5-methoxy-2-methyl-1H-indole | C10 H11 N O | 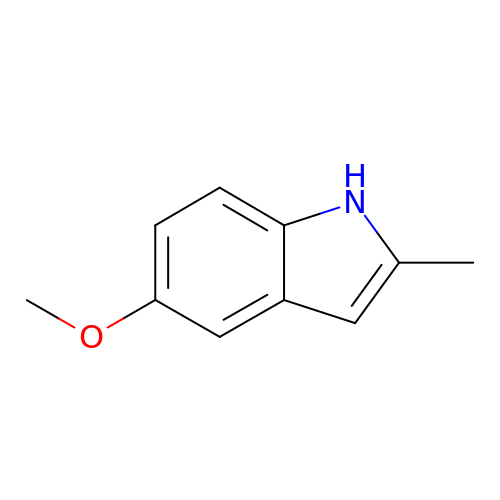VSWGLJOQFUMFOQ-UHFFFAOYSA-N>[2x]GS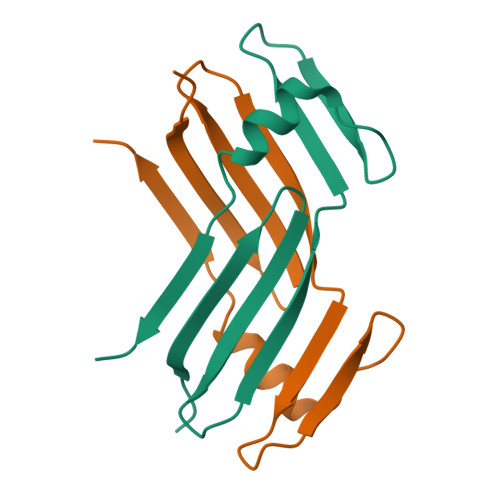AQLLKSVFVKNVGWATQLTSGAVWVQFNDGSQLVMQAGVSSISYTSPDGQTTRYGENEKLPEYIKQKLQLLSSILLMFSNPTPVFQ> MNNGEGEVMDLRDIDLNLLVVFNQLLLDRSVSTAGEKLGLTQPAVSNSLKRLRTALNDDLFLRTSKGMEPTPYALHLAEPVIYALNTLETALTTRDSFDPFASTRTFNLAMTDIGEMYFMPPLMEALAQRAPHIQISTLRPGAGNLKEDMESGAVDLALGLLPELQTGFFQRRLFRHRYVCMFRKDHPSAKSPMSLKQFSELEHVGVVALNTGHGEVDGLLERAGIKRRMRLVVPHFIAIGPILHSTDLIATVPQRFAVRCEVPFGLTT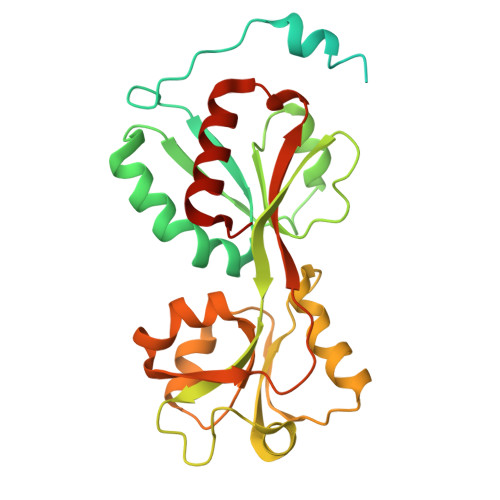SPHPAKLPDIAINLFWHAKYNRDPGNMWLRQLFVELFSEAHHHHHH> MFEITGINVSGALKAVVMATGFENPLSSVNEIETKLSALLGSETTGEILFDLLCANGP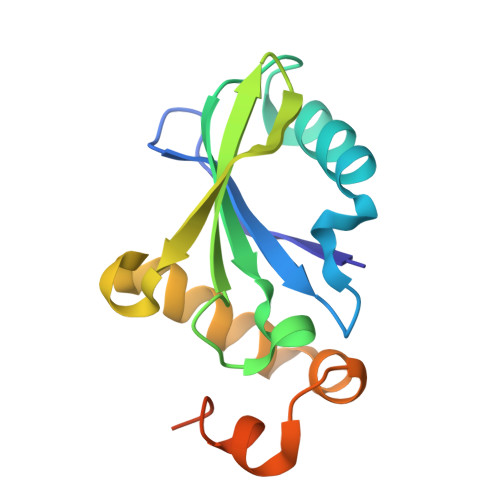EWNRFVTLEMKYGRIMLDTAKIIDEQDVPTHILSKLTFTLRNHPEYLEASVLSPDDVRQVLSMDFAAALEHHHHHH> SSGSSYPSLLQCLKAPVLSDSSCKSSYPGQITGNMICVGFLEGGKDSCQGDSGGP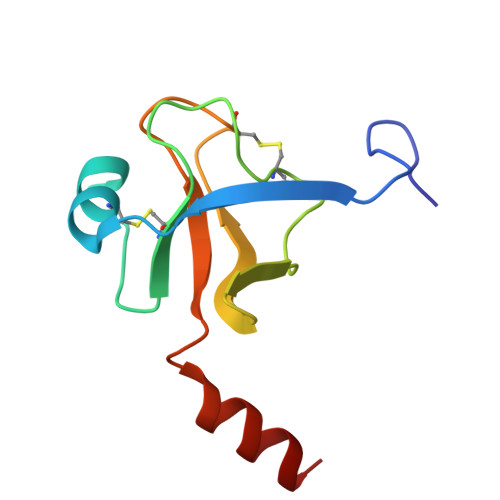VVCNGQLQGIVSWGYGCAQKNKPGVYTKVCNYVNWIQQTIAAN> SLEEGEASSTTSPTEETTQKLTVSHIEGYECQPIFLNVL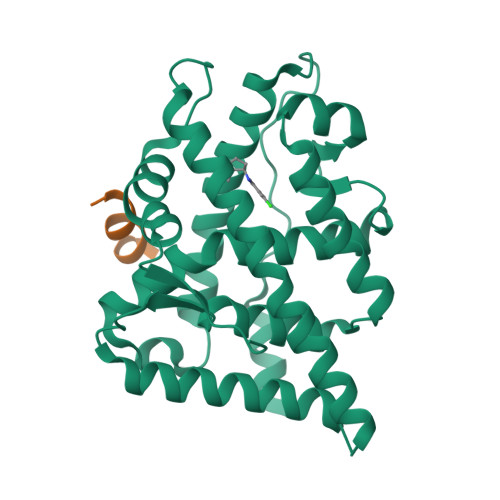EAIEPGVVCAGHDNNQPDSFAALLSSLNELGERQLVHVVKWAKALPGFRNLHVDDQMAVIQYSWMGLMVFAMGWRSFTNVNSRMLYFAPDLVFNEYRMHKSRMYSQCVRMRHLSQEFGWLQITPQEFLCMKALLLFSIIPVDGLKNQKFFDELRMNYIKELDRIIACKRKNPTSCSRRFYQLTKLLDSVQPIARELHQFTFDLLIKSHMVSVDFPEMMAEIISVQVPKILSGKVKPIYFHTQEG;> GAFQNLFQSV>[2x]GSAAATGPSFWLGNETLKVPLALFALNRQRLCERLRKNPAVQAGSIVVLQGGEETQRYCTDTGVLFRQESFFHWAFGVTEPGCYGVIDVDTGKST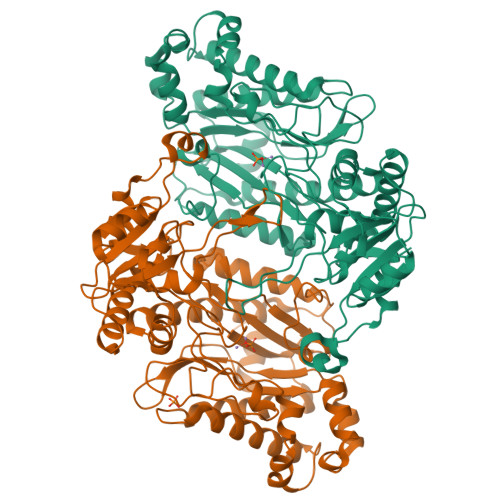LFVPRLPASHATWMGKIHSKEHFKEKYAVDDVQYVDEIASVLTSQKPSVLLTLRGVNTDSGSVCREASFDGISKFEVNNTILHPEIVECRVFKTDMELEVLRYTNKISSEAHREVMKAVKVGMKEYELESLFEHYCYSRGGMRHSSYTCICGSGENSAVLHYGHAGAPNDRTIQNGDMCLFDMGGEYYCFASDITCSFPANGKFTADQKAVYEAVLRSSRAVMGAMKPGVWWPDMHRLADRIHLEELAHMGILSGSVDAMVQAHLGAVFMPHGLGHFLGIDVHDVGGYPEGVERIDEPGLRSLRTARHLQPGMVLTVEPGIYFIDHLLDEALADPARASFFNREVLQRFRGFGGVRIEEDVVVTDSGIELLTCVPRTVEEIEACMAGCDKAFTPFSGPK CYCLOBUTYL(CYCLOPENTYL)FORMAMIDE | C10 H17 N O | 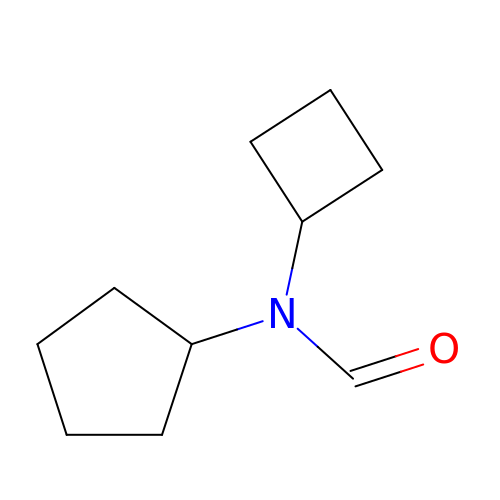DWGVYBRKKSJLNS-UHFFFAOYSA-N>MSHLYDPTTQYYTGEYPKQKQPAPGVQAKMTPVPDCGEKS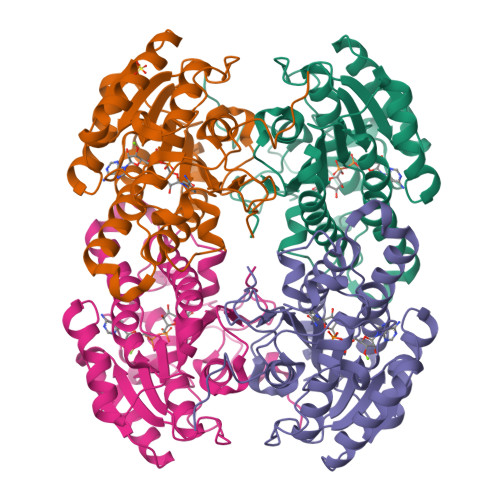YVGSGRLKDRKALVTGGDSGIGRAAAIAYAREGADVAINYLPAEEEDAQQVKALIEECGRKAVLLPGDLSDESFARSLVHKAREALGGLDILALVAGKQTAIPEIKDLTSEQFQQTFAVNVFALFWITQEAIPLLPKGASIITTSSIQAYQPSPHLLDYAATKAAILNYSRGLAKQVAEKGIRVNIVAPGPIWTALQISGGQTQDKIPQFGQQTPMKRAGQPAELAPVYVYLASQESSYVTAEVHGVCGGEHLG[4x]>[4x]VPRGSHMKKLLVANRGEIAVRVFRACNELGLSTVAVYAREDEYSVHRFKADESYLIGQGKKPIDAYLDIDDIIRVALESGADAIHPGYGLLSENLEFATKVRAAGLVFVGPELHHLDIFGDKIKAKAAADEAKVPGIPGTNGAVDIDGALEFAKTYGYPVMIKAALGGGGRGMRVARNDAEMHDGYARAKSEAIGAFGSGEIYVEKYIENPKHIEVQILGDRHGNIIHLHERDCSVQRRNQKVIEIAPAVGLSPDFRNEICEAAVKLCKNVGYVNAGTVEFLVKDDKFYFIEVNPRVQVEHTITELITGVDIVQAQILIAQGKDLHREIGLPAQSEIPLLGSAIQCRITTEDPQNGFLPDTGKIDTYRSPGGFGIRLDVGNAYAGYEVTPYFDSLLVKVCTFANEFSDSVRKMDRVLHEFRIRGVKTNIPFLINVIANENFTSGQATTTFIDNTPSLFNFPRLRDRGTKTLHYLSMITVNGFPGIENTEKRHFEEPRQPLLNLEKKKTAKNILDEQGADAVVDYVKNTKEVLLTDTTLRDAHQSLLATRLRLQDMKGIAQAIDQGLPELFSAEMWGGATFDVAYRFLNESPWYRLRKLRKLMPNTMFQMLFRGSNAVGYQNYPDNVIEEFIRVAAHEGIDVFRIFDSLNWLPQMEKSIQAVRDNGKIAEATICYTGDILDPSRPKYNIQYYKDLAKELEATGAHILAVKDMAGLLKPQAAYRLISELK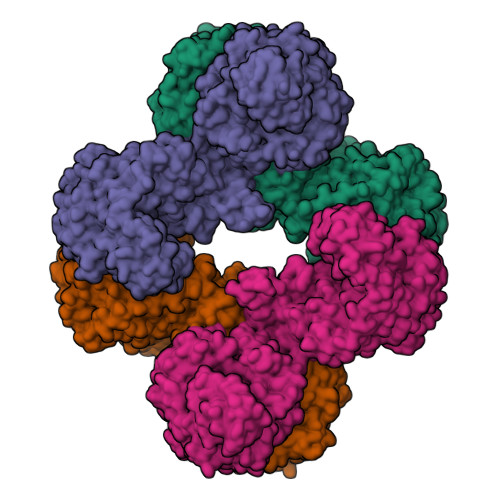DTVDLPIHLHTHDTSGNGIITYSGATQAGVDIIDVATASLAGGTSQPSMQSIYYALEHGPRHASINVKNAEQIDHYWEDVRKYYAPFEAGITSPQTEVYMHEMPGGQYTNLKSQAAAVGLGHRFDEIKQMYRKVNMMFGDIIKVTPSSKVVGDMALFMIQNDLTEEDVYARGNELNFPESVVSFFRGDLGQPVGGFPEKLQKIIVKDKAVITDRPGLHAEKVDFETVKADLEQKIGYEPGDHEVISYIMYPQVFLDYQKMQREFGAVTLLDTPTFLHGMRLNEKIEVQIEKGKTLSIRLDEIGEPDLAGNRVLFFNLNGQRREVVINDQSVQAQVVAKRKAETGNPNQIGATMPGSVLEILVKAGDKVQKGQALMVTEAMKMETTIEAPFDGEIVDLHVVKGEAIQTQDLLIEIN>MPVAGSELQYLGQIQHILRCGVRKDDRTGTGTLSVFGMQARYSLRDEFPLLTTKRVFWKGVLEELLWFIKGSTNAKELSSKGVKIWDANGSRDFLDSLGFSTREEGDLGPVYGFQWRHFGAEYRDMESDYSGQGVDQLQRVIDTIKTNPDDRRIIMCAWNPRDLPLMALPPCHALCQFYVVNSELSCQLYQRSGDMGLGVPFNIASYALLTYMIAHITGLKPGDFIHTLGDAHIYLNHIEPLKIQLQREPRPFPKLRILRKVEKIDD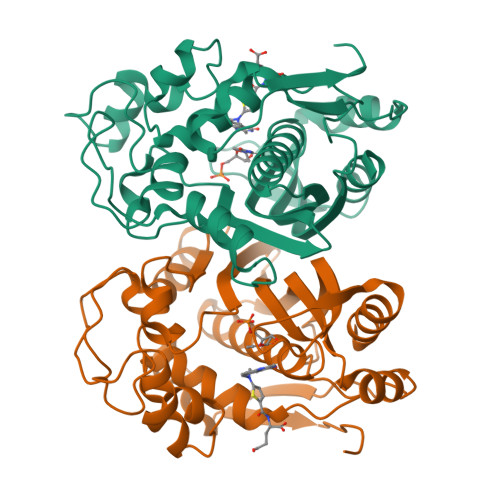FKAEDFQIEGYNPHPTIKMEMAV[2x]> MQRNTYNKVGLYILSLAMLFVFIIILTAKIPFCFTSDCSFIGLKKLVLTNIVPIVCFVFFLFSIYFYNRLKNITKYNGQDSVKITSCQSESYESLTFLATY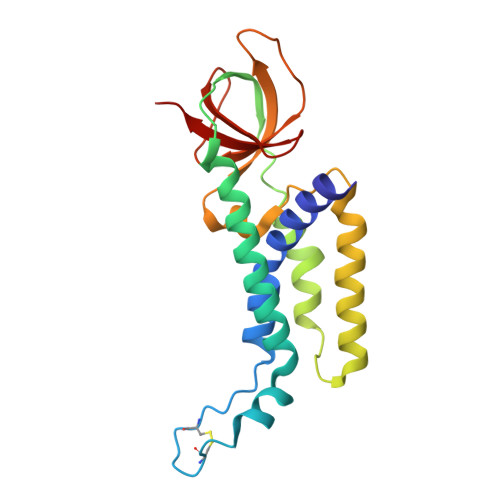IVPFMGFSFEDMQKNIAYLLLVVVIGIIFIKTDKYYANPTLALFGFKLYRVNILHPGSGETKNLIAISNDVLKVDDNVYYSFFDEFVFIARKKI> GSSGSSGDESDNAFIRASRALTDKVTDLLGGLFSKTEMSEVLTEILRVDPAFDKDRFLKQCENDIIPNVLEAMISGELDILKDWCYEAT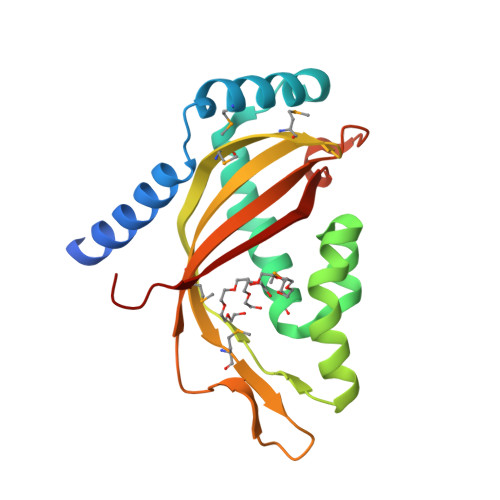YSQLAHPIQQAKALGLQFHSRILDIDNVDLAMGKMVEQGPVLIITFQAQLVMVVRNPKGEVVEGDPDKVLRMLYVWALCRDQDELNPYAAWRLLDISASSTEQIL> MVVLDKKLLERLTSRKVPLEELEDMEKRCFLSTFTYQDAFDLGTYIRNAVKENFPEKPVAIDISLPNGHCLFRTVTYGGSALDN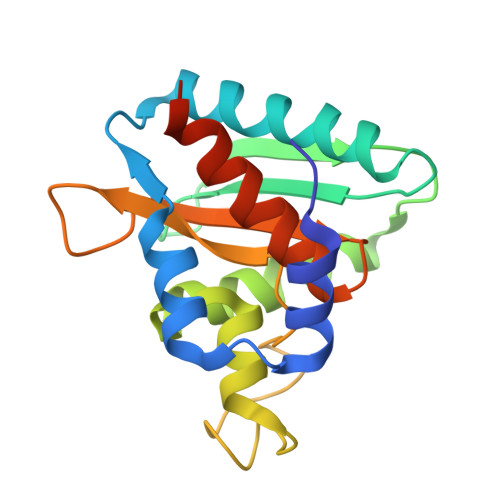DFWIQRKKKTALRFGHSSFYMGCKKGDKTPEEKFFVDSKEYAFHGGAVLIQSERSDYPYACLTISGLKQEEDHLMALSSLIAFANESLEEDLNLD> AGTKLSLMPWFHGKITREQAERLLYPPETGLFLVRESTNYPGDYTLCVSSD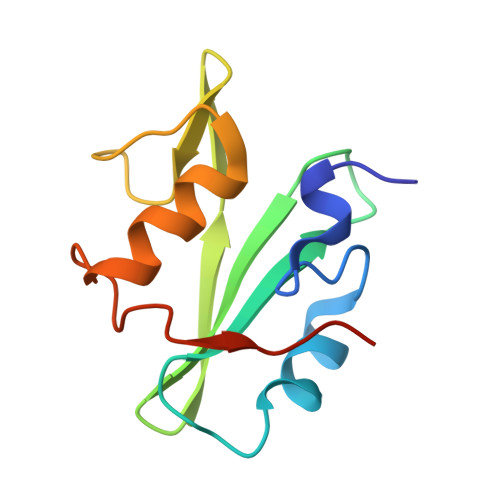GKVEHYRIMYHASKLSIDEEVYFENLMQLVEHYTSDADGLCTRLIKPKVMEGTVA> DISSTE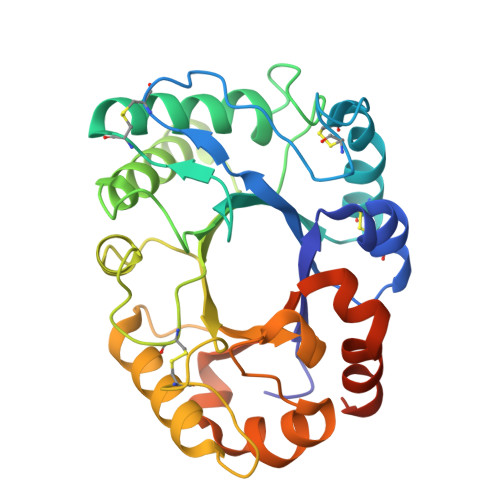IAVYWGQREDGLLRDTCKTNNYKIVFISFLDKFGCEIRKPELELEGVCGPSVGNPCSFLESQIKECQRMGVKVFLALGGPKGTYSACSADYAKDLAEYLHTYFLSERREGPLGKVALDGIHFDIQKPVDELNWDNLLEELYQIKDVYQSTFLLSAAPGCLSPDEYLDNAIQTRHFDYIFVRFYNDRSCQYSTGNIQRIRNAWLSWTKSVYPRDKNLFLELPASQATAPGGGYIPPSALIGQVLPYLPDLQTRYAGIALWNRQADKETGYSTNIIRYLNATAMPFTSNLLKYPS N-[(1R,2S)-1-[(2R,4R)-4-(cyclohexylmethoxy)pyrrolidin-2-yl]-3-(3,5-difluorophenyl)-1-hydroxypropan-2-yl]acetamide | C22 H32 F2 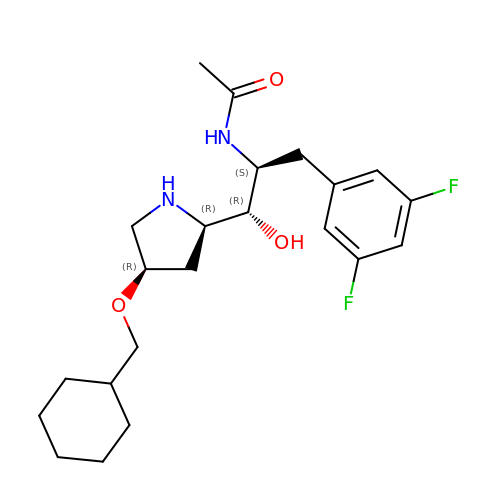N2 O3 | MSAOCNJMXAZEEN-YUMYIRISSA-N> MLKQVEIFTAGSALGNPGPGGYGAILRYRGREKTFSAGYTRTTNN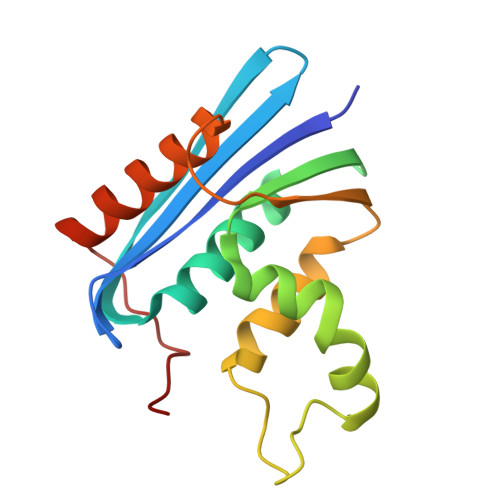RMELMAAIVALEALKEHAEVILSTDSQYVRQGITQWIHNWKKRGWKTADKKPVKNVDLWQRLDAALGQHQIKWEWVKGHAGHPENERADELARAAAMNPTLEDTGYQVEV> SFWEWLNAVFNKVDHDRIRDVGPDRAASEWLLRCGAMVRYHGQQRWQKDYNHLPTGPLDKYKIQAIDATDSCIMSIGFDHMEGLQYVEKIRLCKCHYIEDGCLERLSQLENLQKSMLE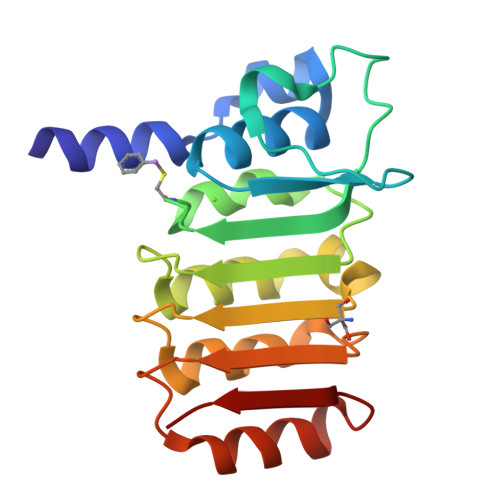MEIISCGNVTDKGIIALHHFRNLKYLFLSDLPGVKEKEKIVQAFKTSLPSLELKLDLK Bacteriophage Casadabanvirus JBD30, from the order Caudoviricetes, is a temperate phage that infects the bacterium Pseudomonas aeruginosa. The virion of bacteriophage JBD30 is composed of an icosahedral capsid, long flexible non-contractile tail, and a baseplate. Using its baseplate, JBD30 attaches to Pseudomonas aeruginosa via the bacterial type IV pilus, whose subsequent retraction brings the phage to the bacterial cell surface.

The core of the baseplate is formed of a trimer of baseplate hub proteins (gp53). The shape of the baseplate hub protein trimer resembles a trophy cup, as it was termed for phage T5. The baseplate hub protein is composed of seven domains. Domain IV forms an interface for binding to distal tail proteins and gives rise to a long linker, which spans the whole baseplate hub monomer. The tip of the baseplate is closed by three α-helices, each protruding from one baseplate hub domain V. Besides playing the role of a baseplate organiser, the trimer of baseplate hub proteins also provides attachment sites for the tail fibres and receptor-binding proteins. The upper baseplate protein (gp50) is composed of two domains, each formed of a central β-sandwich with an α-helix, connected by a flexible linker. Domain I of the upper baseplate protein sits in a gap between the domain IVs of two baseplate hub proteins. The upper baseplate protein domain II is attached to the surface of the baseplate hub domain III. Residues Cys147, Cys156, Cys238, and Cys245 coordinate a putative metal ion in domain II of the upper baseplate protein.

> MATFPGFQVPKPVEGIVAGITPNIDALELNQDISLAAVAASTWGGAYGAHQPVEVIHSTYQAVHQSALEENYYNRLWLIPTAMELGNVVSTQIRPASVWNAYFSPRTLTAIDREAADGITLSGQASPPLGFAALEERTWTVSIGTDGPPVVNARIVWRLQGEPNLVLVITGNRIIAWTFAPDWGDSIVERLSASTNILQSESAVTQRRAMRLAPRREFDANMYAVDRERQLLDMTLFGWGARIWALPIWPDIQLLHQPLAAGSLGIPCDTAGLDFRDGGLAMLRGEDAFTYEVVEVKTVTASGLDLVRPVQAAWGTGSRLYPVRTAQLTEQPTLTRLTDTAQSARVSFLVMEPSAWPELMPATTYRGRPVLEQRPDESEDLTSSYQRLLSTLDNGSAIPRVTDVAGMALPVIGHRWIGMGRAERSAFRSLVYALRGQQKPLWVPTHADDLTLVATVSQLSTALDVRNIGYARFANGRPGRRDIRIELYDGTVYHRRILTSTELDADTERVAIDAALGRLVEPTDVARICFMALCSAASDVVEIEHVTDSEGVATAALTFKGVRDDEF;> MSFNSRESSLADGQPVRLYQFSRGAIRWSYNSSDRDITYQNQIFRTVPGGITDNGIICSGDPQSDQFVITAPADLDVALLYKTRSPSDAIDLVVYDMHYGDAEAAVSWVGQIGDVDWPTVDSCRITCVSEDELMDQPGLTDTYCRTCTAIVGDHRCKVNLVPYRVTLTPQSVSAWVISSGVVAGYADGWFTGGYVEWQVDGDNYDRRFIEQHAGADLHILGGTEGIPAGGQLRVYPGCDGLAQTCDDKFSNLPNFRGFNAMQGKSPFDGDQVW;> MGAKPKAQTVGWRYYFDIHFALGKKVDEVCAIRASGKTAWKGSITSNGQVRINAPELFGGDKGEGGLDGTLDVLFGEEDQGVLPRLAAMLGGLVPAFRGVTTCFYSGLVTSVNPYPKKWEILRRGGNRLWDGNPWYPEKQFVWLADGQIKAMNPAHILYLVYTGRDFRGLARTRMDEASWRAAADTLYAEGFGLCFEWTRSDSFKNFCETVKSHIGAEVYPNRQTGQISIRLLRDDYNVADLPLFDEDSGLLEITQEKTGSTSLAPSQLIVKYIDQIDGAQRQIIVNNNAVAASQGRRSSEEIEFLGVPTGELAGRVGEREMRLKTTGLKRYKGVFDRRARSLNPGQPFLIRSTPRGIPETVVRVGRIEDNFLGDGKITLTVVQDQFNLPATTGVAPPPPGWTPPDRTPRAITVRRLIEAPYRELAGVIDPANLQLLDVSASYLAALAEAPTSLSQSYTLTDRVGSSGAFVDRGTGDWCPTGLLAAELPLAAGPNVVTLTNATRLEDVTVGQAAVVDDEIVRVDAVNYASGTVTLARGCADTVPAKHLAGARVWFYDTFEAVDETVYSQGVTLQARLLTNTSEGQLAPALAATDSLTLTGRQGKPYPPGQFRINGSAYPTKVYGALSVSWAKRDRIGQADQLIDTTVGNIGPEDGATVTLQVYSGTTLKRTYAGLTSSSWSYPLAEDMADGPLQDVRLVLRSVRDGIDSWQQHDITIERHGLGFRLGEELGGVSA> SGISLDNSYKMDYPEMGLCIIINNKNFHKSTGMTSRSGTDVDAANLRETFRNLKYEVRNKNDLTREEIVELMRDVSKEDHSKRSSFVCVLLSHGEEGIIFGTNGPVDLKKITNFFRGDRCRSLTGKPKLFIIQACRGTELD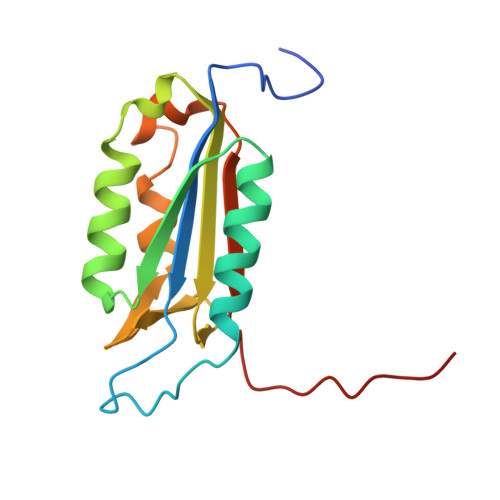CGIET The transcriptional activity of the HIFs is regulated in an oxygen dependent manner by 2-oxoglutarate (2OG) and ferrous iron dependent oxygenases which catalyze the post-translational hydroxylation of HIF-α subunits. Two proline-residues, Pro402 and Pro564 in human HIF-1α, in the N- and C-terminal regions of the oxygen-dependent degradation domains, termed NODD and CODD, respectively, of HIF-α isoforms are efficiently hydroxylated by the HIF prolyl hydroxylases (PHDs or EGLNs) under normoxic conditions. In a second 2OG oxygenase-mediated mechanism of HIF regulation, factor inhibiting HIF (FIH) regulates HIF transcriptional activity via 2OG dependent hydroxylation of an asparagine-residue in the C-terminal transcriptional activation domain (CTAD) of HIF-α isoforms; such reaction reduces binding of HIF to transcriptional co-activator proteins (CBP/p300), which are histone lysine acetyltransferases. Here we report studies that inform on the activities, mechanisms of action, and selectivities of the PHD inhibitors (and related compounds) in clinical trials for anaemia treatment, i.e. Vadadustat from Akebia Therapeutics currently in phase III, FG-4592 from FibroGen in phase III, GSK1278863 from GlaxoSmithKline in phase III, and Molidustat from Bayer in phase II.

R8J, has the same tricyclic core as Molidustat and coordinates the metal in PHD via the nitrogens of its pyrazolone ring (trans to Asp-315) and pyridine (trans to His-374) ring; its triazole ring is positioned to from electrostatic interactions with the 2OG binding residue Arg-383, i.e. the triazole ring of Molidustat occupies the same site as the glycinamide side chain of FG-4592/FG-2216. Surprisingly, analysis of Molidustat complexed with FIH (for which it is a poor inhibitor) reveals that the nitrogen of its pyrimidine ring is positioned to ligate to the metal trans to the distal histidine, as do R8J and 2OG in binding to PHD2 and not trans to the proximal histidine, as observed for FIH-2OG binding (Fig. S2†). Thus, the binding mode of Molidustat to FIH might in this respect reflect that of Molidustat to PHD2. A model of the PHD2.Mn.Molidustat complex based on overlay of FIH.Zn.Molidustat and PHD.Mn.R8J structures indicates that the Molidustat morpholine ring may not completely block substrate binding, consistent with NMR studies (see below). In the deacetoxycephalosporin-C synthase (DAOCS) subfamily, of which the PHDs are members, the 2OG C-1 carboxylate (normally) coordinates trans to the distal (i.e. C-terminal) iron-chelating histidine, whereas for Jumonji C (JmjC) subfamily members (of which FIH is a member) it is (normally) trans to the proximal (i.e. N-terminal) histidine of the HxD···H motif.

> SMAATAAEAVASGSGEPREEAGALGPAWDESQLRSYSFPTRPIPRLSQSDPRAEELIENEEPVVLTDTNLVYPALKWDLEYLQENIGNGDFSVYSASTHKFLYYDEKKMANFQNFKPRSNREEMKFHEFVEKLQDIQQRGGEERLYLQQTLNDTVGRKIVMDFLGFNWNWINKQQGKRGWGQLTSNLLLIGMEGNVTPAHYDEQQNFFAQIKGYKRCILFPPDQFECLYPYPVHHPCDRQSQVDFDNPDYERFPNFQNVVGYETVVGPGDVLYIPMYWWHHIESLLNGGITITVNFWYKGAPTPKRIEYPLKAHQKVAIMRNIEKMLGEALGNPQEVGPLLNTMIKGRYN(2R)-2-[3-chloro-4-(methylsulfonyl)phenyl]-3-[(1R)-3-oxocyclopentyl]-N-(pyrazin-2-yl)propanamide 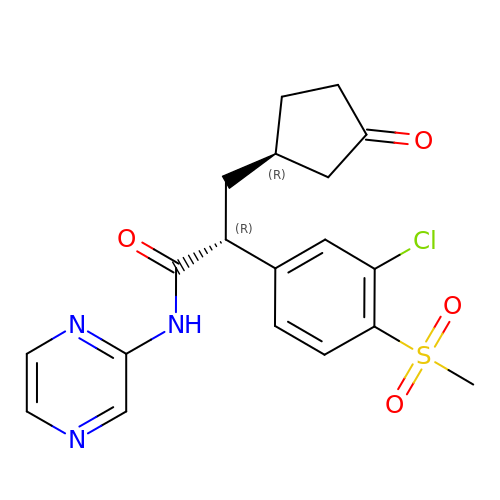| C19 H20 Cl N3 O4 S | XEANIURBPHCHMG-SWLSCSKDSA-N> MDQETIDTDYDVIVLGTGITECILSGLLSVDGKKVLHIDKQDHYGGEAASVTLSQLYEKFKQNPISKEERESKFGKDRDWNVDLIPKFLMANGELTNILIHTDVTRYVDFKQVSGSYVFKQGKIYKVPANEIEAISSPLMGIFE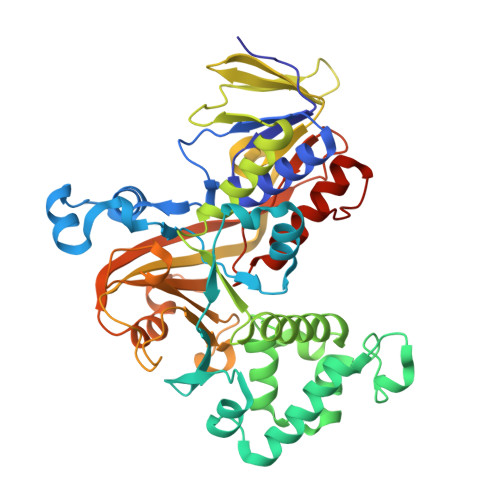KRRMKKFLEWISSYKEDDLSTHQGLDLDKNTMDEVYYKFGLGNSTKEFIGHAMALWTNDDYLQQPARPSFERILLYCQSVARYGKSPYLYPMYGLGELPQGFARLSAIYGGTYMLDTPIDEVLYKKDTGKFEGVKTKLGTFKAPLVIADPTYFPEKCKSTGQRVIRAICILNHPVPNTSNADSLQIIIPQSQLGRKSDIYVAIVSDAHNVCSKGHYLAIISTIIETDKPHIELEPAFKLLGPIEEKFMGIAELFEPREDGSKDNIYLSRSYDASSHFESMTDDVKDIYFRVTGHPLVLKQRQEQEKQ We characterized CtGH76 from the sordariomycete Chaetomium thermophilum, a member of the Fungi/Bacteria-mixed GH76 subfamily, revealing conserved structural features and functional divergence within the GH76 family. Notably, our structural characterization by X-ray crystallography combined with glycan fragment screening indicated that CtGH76 can recognize GPI-anchors like members of the Dfg5 subfamily but shows a broader promiscuity toward other glycans with central α1,6-mannobiose motifs due to the presence of an elongated glycan-binding canyon. Here, we present the crystal structure of a novel fungal GH76 member from the F/B-mixed subfamily, in complexes with different glycans and glycan fragments. Together with structural bioinformatics, we found that members of the F/B-mixed subfamily act as secreted GHs in glycan degradation, which includes not only α1,6-mannans but also GPI-core glycans. Compared to other GH76 orthologs, our findings demonstrate that CtGH76 features an elongated glycan-binding canyon, adept at accommodating a wider range of complex glycans.

CtGH76 crystals belong to space group P3121 with unit-cell parameters of a = 106.8, b = 106.8, c = 126.9 Å, α = β= 90°, and γ = 120° and one molecule per asymmetric symmetry unit. Accordingly, CtGH76 shares the same DD-motif, D163/D164 (black dashed box), in its active site as BcGH76 from Bacillus circulans TN-31 (D124/D125) and CtDfg5 (D134/D135). For Bt3792, the GH76 enzyme from Bacteroides thetaiotaomicron VPI-5482T, these two neighboring aspartate residues were shown to participate in substrate hydrolysis via a retention mechanism. Furthermore, the active site and the canyon-like glycan binding site of CtGH76 is lined with seven aromatic amino acids (W110, W111, W149, Y217, W287, Y289, F352) that potentially interact with the substrate (Figure 2, red dashed box; for nomenclature, refer to Vogt et al.), within an otherwise mostly negatively charged canyon. The tertiary structure of CtGH76 is stabilized by two disulfide bridges (blue dashed box), C204–C279 and C339–C345. C204 anchors the loop connecting helices α5 and α6 via its disulfide bridge to β-sheet β1, whereas the second disulfide bridge, C339–C345, is situated within the loop connecting helices α9 and α10. CtGH76 features two wing-like β-hairpins protruding between helices α7 and α8 (β1/2, D268-R283, designated as WR1) and between helices α11 and α12 (β3/4, R396-D413, WR2). Only WR1 apparently elongates the glycan-binding canyon for providing additional sites of interactions with longer substrates. Otherwise, the CtGH76 resembles other structurally known members of the GH76 family. Compared to the fungal CtDfg5 paralog, CtGH76 exhibits an r.m.s.d. of 1.31 Å over 299 aligned Cα atoms and includes an additional short α-helix (α13).

> MAGIADLTAALASADRNRVTRVEAMRRSPTTISLSTLGALSALWGILYFMTCSGRNSRGVLADASSGMLQTRQSDSESLNSTGLAQAAINGLNARFYESSNARWSSDEPWWISGVALTMVIEYMRRSGSKEYLDQVEDVIEVQRQPLSWWPSGEGEFRADATDDTGWWALAMVRMYDLTGNEDYLNISIKDEAYMRQWWTDTECGGGLYVDIQDLTYKNAIANELYLKLVASLANRAPNATIYLDRAQQAWTWFLGSGMINGVNLINDGLARDSNTGSCYNNRLPVWTYNQGVILGALVELYHATKDESYLLSAQAIADAVLSPSNGLTSSSGVLTETCEGSDSCNQDQQVFKGVFALNLAELGDAVAGASSDPDAGQDYREYLDTNMQSMYANDRSEIVPTLFDSSTGDLYDVSWSGPFRNATMPKQASAIGLYVANI>[2x]MELKPNVKEIPGPKARKVIEEHHKYMATTTNDPNEYFLVIERAEGVYWIDVDGNVLLDFSSGIGVMNVGLRNPK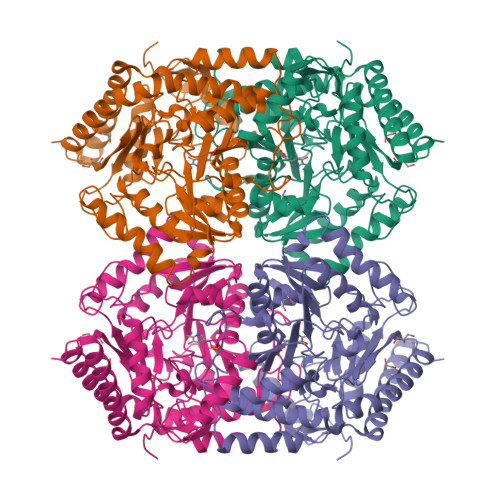VIEAIKKQLDLVLHAAGTDYYNPYQVELAKKLVEIAPGDIERKVFLSNSGTEANEAALKIAKWSTNRKMFIAFIGAFHGRTHGTMSLTASKPVQRSRMFPTMPGVVHVPYPNPYRNPWGIDGYENPDELINRVIDYIEEYLFEHYVPAEEVAGIFFEPIQGEGGYVVPPKNFFKELKKLADKHGILLIDDEVQMGMGRTGRMWAIEHFDIVPDIVTVAKALGGGIPIGATIFRADLDFGVSGVHSNTFGGNTVAAAAALAVIEELQNGLIENAQKLEPLFRERLEEMKEKYEIIGDVRGLGLAWGVEFVKDRKTKEYATKERGEIVVEALKRGLALLGCGKSAIRLIPPLIISEEEAKMGLDIFEEAIKVVSERHGYKIH>[2x]MSVLTVPRQTPRQRLPVLPCHVGDPDMWFADTPAGLEVAKTMCVSCPIRRQCLAAALQRAEPWGVWGGEIFDQGSIVSH;>MAHHHHHHVAVDA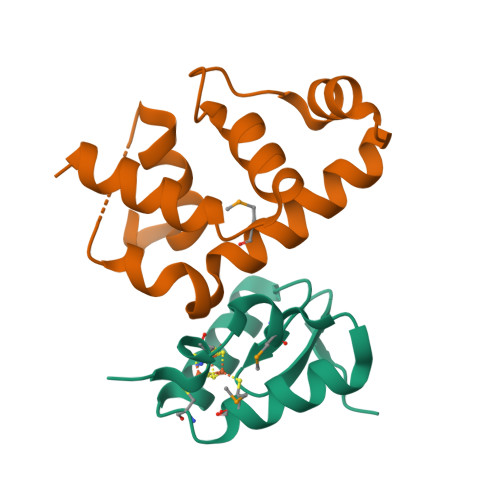VSFTLLQDQLQSVLDTLSEREAGVVRLRFGLTDGQPRTLDEIGQVYGVTRERIRQIESKTMSKLRHPSRSQVLRDYLDGSSGSGTPEERLLRAIFGEKA[2x]>RNLMIVDGTNLGFRFKHNNSKKPFASSYVSTIQSLAKSYSARTTIVLGDKGKSVFRLEHLPEYKGNRDEKYAQRTEEEKALDEQFFEYLKDAFELCKTTFPTFTIRGVEADDMAAYIVKLIGHLYDHVWLISTKGDWDTLLTDKVSRFSFTTRREYHLRDMYEHHNVDDVEQFISLKAIMGDLGDNIRGVEGIGAKRGYNIIREFGNVLDIIDQLPLPGKQKYIQNLNASEELLFRNLILVDLPTYCVDAIAAVGQDVLDKFTKDILEIAE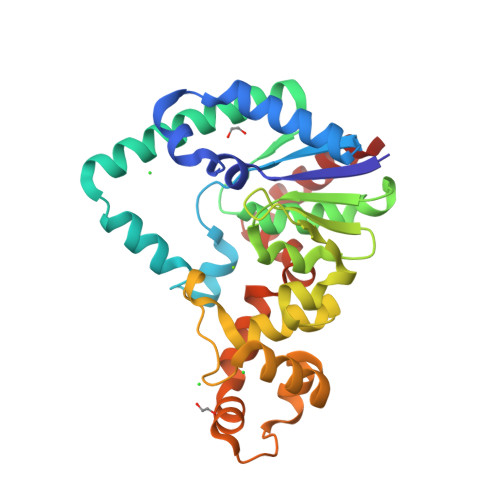Q[2x]> PGTSIEWHKFETSEEIISTYLIDDVLYTGVNGAVYTFSNNELNKTGLTNNNNYITTSIKVEDTLV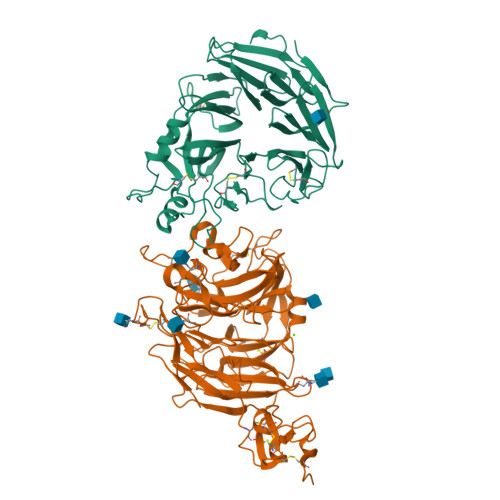CGTNNGNPKCWKIDGSEDPKYRGRGYAPYQNSKVTIISHNECVLSDINISKEGIKRWRRFDGPCGYDLYTADNVIPKDGVRGAFVDKDGTYDKVYILFTDTIDTKRIVKIPYIAQMCLNDEGGPSSLSSHRWSTFLKVELECDIDGRSYRQIIHSKAIKTDNDTILYVFFDSPYSKSALCTYSMNAIKHSFSTSKLGGYTKQLPSPAPGICLPAGKVVPHTTFDIIEQYNELDDIIKPLSQPIFEGPSGVKWFDIKEKENEHREYRIYFIKENTIYSFDTKSKQTRSAQVDARLFSVMVTSKPLFIADIGIGVGIPRMKKILKM;> ADEPVWRSEQAIGAIAASQEDGVFVASGSCLDQLDYSLEHSLSRLYRDQAGNCTEPVSLAPPARPRPGSSFSKLLLPYREGAAGLGGLLLTGWTFDRGACEVRPLGNLSRNSLRNGTEVVSCHPQGSTAGVVYRAGRNNRWYLAVAATYVLPEPETASRCNPAASDHDTAIALKDTEGRSLATQELGRLKLCEGAGSLHFVDAFLWNGSIYFPYYPYNYTSGAATGWPSMARIAQSTEVLFQGQASLDCGHGHPDGRRLLLSSSLVEALDVWAGVFSAAAGEGQERRSPTTTALCLFRMSEIQARAKRVSWDFKTAESHCKEGDQPERVQPIASSTLIHSDLTSVYGTVVMNRTVLFLGTGDGQLLKVILGENLTSNCPEVIYEIKEETPVFYKLVPDPVKNIYIYLTAGKEVRRIRVANCNKHKSCSECLTATDPHCGWCHSLQRCTFQGDCVHSENLENWLDISSGAKKCPGAP> FFYYRFHKRIGKGNFNRYLEFYQKPRGIENTLRLRYNYTPTFTAKKRSEMWKVNLVKKIAHATDAKQVLDVWTYYRHRRTKRPYHYLLALQRLVEVGGCDPTDFRFRLIARGIYRTAKRFINLPRVCVYLAKLNATGDLQDLSRFLIPQVEAYFPFQLCLLAHAFGSVRLQDKVLFAAIDEALRPHLSELPAAMLVKLTQGYAGALVHNYGLLARVSLLLQQRLSRAATGEADPLTACDEEDETGRTLSSKEPQGGSRQRETTKAAREITEAEDDCLEATEKKTVKRRHSGPLLPTLHHLLAFGRVCADLKYQDFGYLEMLSIQMQAAFRADLAVSSSRETFQRFSPFSVQELVEIFHRLK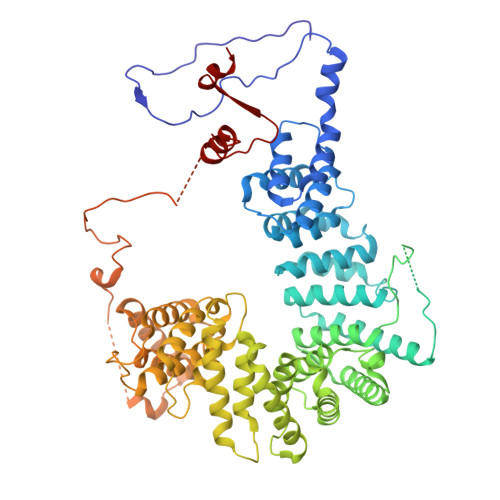VNDVSLLLAALRHVQARMHDYPPSCVASIGFCTAQMLPCDASTVRQVHAQMLEVLQEAVPLLDLCSLGQLAAFAKKAKPRRNRSALRSSVFEAVEARVIELQGDGRTVFDVGRLLELLSLNGRRVSEEAFHILCRQAHRHLDLFEPQDFCRLARALARVKCQGSRGEQSEGLQASSLVNALARRTLRQEDEFSPRDFLSLLRSLTLAGPPDRVYAVPLKEKLRRKQVLHNYFPASQSEDAEAFEDSEQLLESDLPPSSRQTPTLRKGRLLLGPQVIRRPQQQGSPESAEGEARSEKETLEEESLSYSPVPDGEQEAEVNGNHAGKSVSVLSEGGRSRIRRRRLEEKLRIAEEEGWDLLHRRVASLRQLKGWL>MISGWGARPEEQYEMIRAAVPPSEAEPRLQEALVVVNALLPAPITLDDALGSLDDTRRLVKARALARTYHACMVNLERLARHHPGLEAPTIDGAVAAHQDKMRRLADTCMATILQMYMSVGAADKSADVLVSQAIR[4x];>[4x]MAAATADDEGSAATILKQAIAGDRSLVEAAEAISQQTLLRLACEVRQVGDRQPRFTATSIARVDVAPGCRLRFVLDGSPEDAYVTSEDYFKRCCGQSSYRGFAVAVLTANEDHVHSLAVPPLVLLHRFSLFNPRDLLDFELACLLMYLENCPRSHAT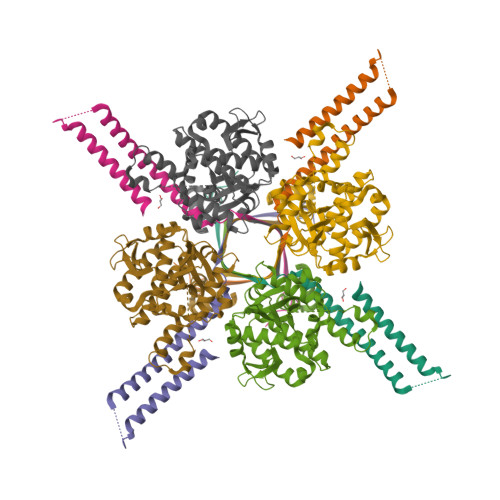PSTFAKVLAWLGVAGRRTSPFERVRCLFLRSCHWVLNTLMFMVHVKPFDDEFVLPHWYMARYLLANNPPPVLSALFCATPTSSSFRLPGPPPRSDCVAYNPAGIMGSCWASEEVRAPLVYWWLSETPKRQTSSLFYQFCGSLEVLFQ>GAMGMGLAGGSLPSLAPDLVRDLIATAADISLLVSQEGVVREVMANPHHPSFGQLSEWEGRPLEEVLTAESVAKFRLRSEGLEPGRGSVAVELNHIDPRSFEFPIRYILHRLPADRSILMLGRDLRPIAEVQQQLVAAQLAMERDYETQREMETRYRVVLDVSRDPMVLVSMSTGRIVDLNSAAGLLLGGVRQDLLGAAIAQEFEGRRRGEFMETMTNLAATESAAPVEVLARRSQKRLLVVPRVFRAAGERLLLCQIDPAD[2x];> VEADTFALYALTEAQA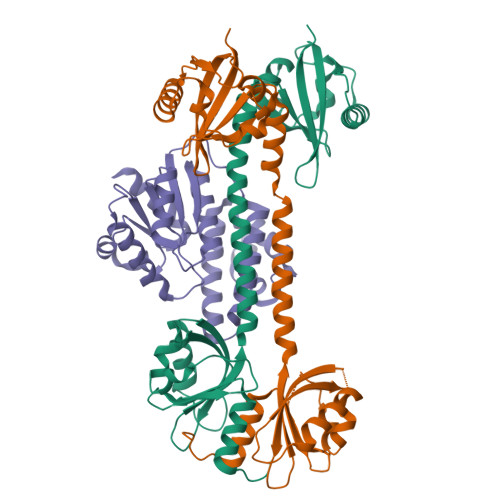GRSGRAKAVARLSDLLSTDPLGRLTEVEELLRAHAPTAADFARLFEACAERLTRALAEDRISRMQVTLAYSALQMALRRIHHLPDPQKSVGAVLVAGVPGHKPILEAALAAEMLRAVGWSTSVVHPESVAALAARLKTSRTSTLVVAPSLLEGTEQEADTLRFVSALRARTDLPGLSILVGGRLAQLPPSKLKDSGADAGFAHLALLPAALARVASSAHHHHHH>[2x]MGSSHHHHHHSSGLVPRGSHMSNQNAPTPPPTEVIQLDWWKNCVLYQIYPRSFKDSDGDGIGDLKGIISELKHFVDAGVDAIWMSPIFESPMVDFGYDISNFYDIHYEYGTMEDFEELLDKAHELGLKVLLDFVPNHASNESEYFIKSEAREPGYENFFIWADPLPNPENPGVRLPPSNWVSQFGGSAWEWSEKRQQYYLHQFAIQQVDFDFRNPAVKQEMFNIMKFWLDKGADGFRLDALPYLIEADPADHEGRYPDDPLSGLTQFESHQLGYTIPLYTKDLIELYDVVYEWREFLDEYNKNHGGDTRVVFSQGYANVSMTMLYYGNEDGAIGAHFPFNFDFITDLSSKSNARDFVYIILRWLTYMPYGGIPNWVFGNHDNNRMPTRFRHDMV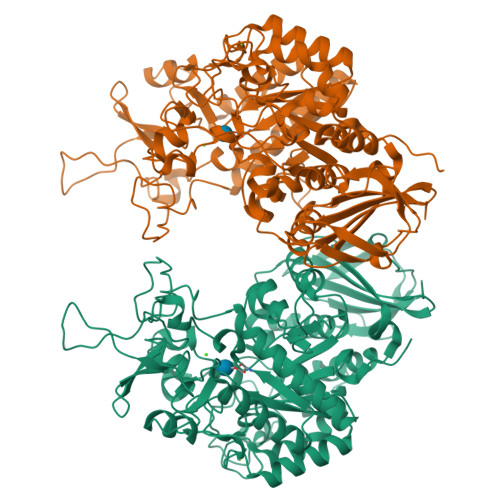DGLNIINMLLPGVAVTYQGEEIGMRDGYVSWEDTVDIEACNRGDPDTYHLYSRDPARTPYHWDNSTSAGFSTSTNTWLPVAEDYQEINLAKQKETARSHFKNYQALTKLRKQATLSHGEYDIRALSDRTFYLVRSLPTHDTYVLLFNVSERRDTVDLGRVPHLTLPATVYVSSIHSARLAGHEITSSQLSLEAGEALVLKAQPI>[2x]MQTEHVILLNAQGVPTGTLEKYAAHTADTRLHLAFSSWLFNAKGQLLVTRRALSKKAWPG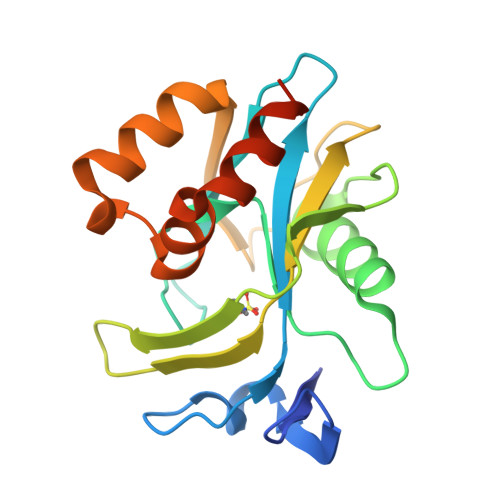VWTNSVAGHPQLGESNEDAVIRRCRYELGVEITPPESIYPDFRYRATDPSGIVENEVCPVFAARTTSALQINDDEVMDYQWCDLADVLHGIDATPWAFSPWMVMQATNREARKRLSAFTQLKLEHHHHHH>PMFIVNTNVPRASVPDGFLSELTQQLAQATGKPPQYIAVHVVPDQLMAFGGSSEPCALCSLHSIGKIGGAQNRSYSKLLCGLLAERL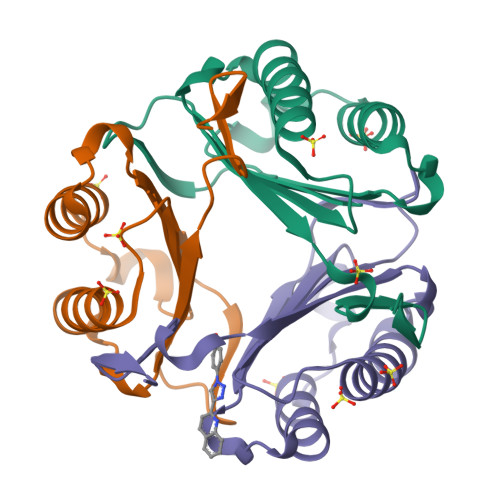RISPDRVYINYYDMNAANVGWNNSTFA[18x]> MAAPLGGMFSGQPPGPPQAPPGLPGQASLLQAAPGAPRPSSSTLVDELESSFEACFASLVSQDYVNGTDQEEIRTGVDQCIQKFLDIARQTECFFLQKRLQLSVQKPEQVIKEDVSELRNELQRKDALVQKHLTKLRH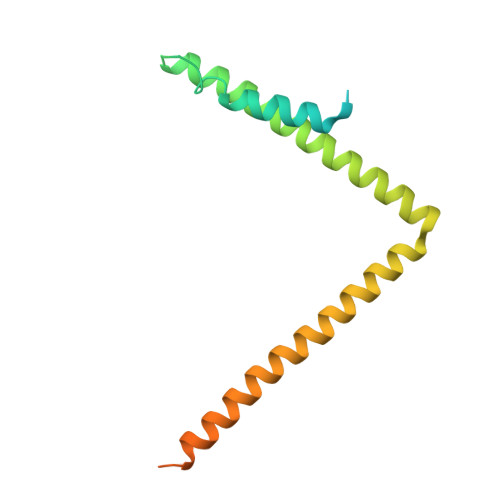WQQVLEDINVQHKKPADIPQGSLAYLEQASANIPAPLKPT Several natural systems exhibit ‘facilitated dissociation’, in which an effector (E) can bind to a target–host (TH) complex to form an excited ternary complex (THE)20–26 from which the target dissociates quickly. We set out to design protein systems that undergo facilitated dissociation. We use a switchable target binder (host) and a flexible effector that can rapidly bind to and switch the target–host complex to induce a large steric clash with the target, forming a strained excited ternary complex. We show here that by explicitly considering excited intermediate states when designing coupled protein systems, a broad range of facilitated dissociation systems can be designed.

To allosterically couple binding of the effector to dissociation of the target, we designed structured fusions of the hinge switch and binder such that when the switch is in state X, the target can bind, but when in the effector-bound state Y, it will clash strongly. To measure facilitated dissociation kinetics, we used surface plasmon resonance (SPR): with the target affixed to the SPR surface, we incubated with the host, then measured target–host dissociation under flow of various concentrations of effector. For these four designs, the target dissociates slowly in the absence of the effector; adding the effector increases the rate of dissociation markedly, but minimally affects the target off-rate from a control static binder fusion that lacks an effector-binding site.

>[2x]MSGEEAVRRRFEELLREALAFRERTGGRRETLEHAVRLARELAEFAASHPEFNRQEAVLLAIELMVRAMGVTMETHRSGNEVKVVIKGLNIDEQRALYRAVRETSKIMGVETEIEVEGDTVTIVVREGSG>[4x]EPDIRPCGRSLVIISTLDGRIAALDPENHGKKQWDLDVGSGSLVSSSLSKPEVFGNKMIIPSLDGDLFQWDRDRESMETVPFTVESLLESSYKFGDDVVLVGGKSLTTYGLSAYSGKVRYICSALGCRQWDNDEMEQEEDILLLQRTQKTVRAVGPRSGNEKWNFSVGHFELRYIPDMETRAG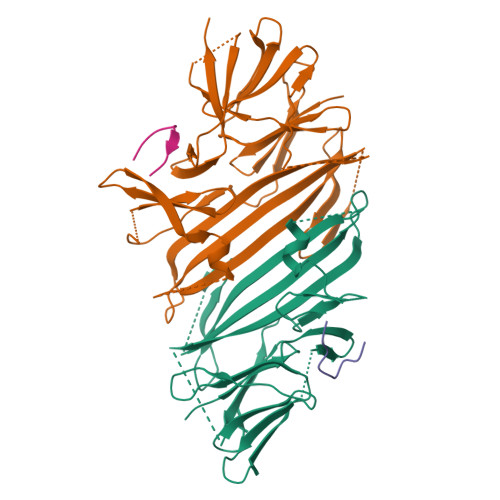FIESTLKPSGNKEQSKIISDVEEQEAVMMDTVIKVSVADWKVMAFNKKGGHLEWEYQFSTPIASAWLVKDGKVIPISLFDDTSYAPNDGVLEDEEDIVEAARGATENSVYLGMYRGQLYLQSSVRISEKFPTSPKALESVSSE;>ADPQPWRFYAPR[3x]> MARRKCRNRFVKKNGQCNVEFTNMDDWPQRYIADMFTTCVDIRWRYMLLLFSLAFLVSWLLFGLIFWLIALIHGDLENPGGDDTFKPCVLQVNGFVAAFLFSIETQTTIGYGFRCVTEECPLAVFMV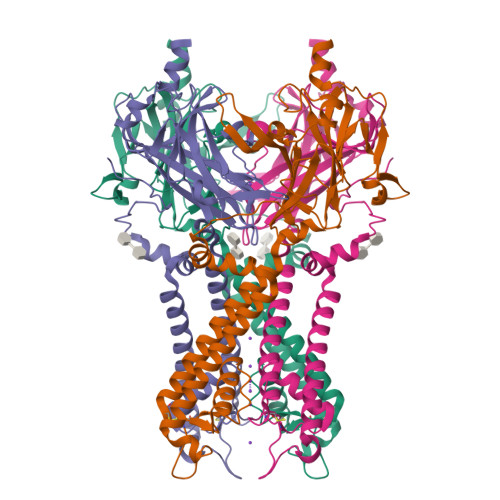VVQSIVGCIIDSFMIGAIMAKMARPKKRAQTLLFSHNAVVAMRDGKLCLMWRVGNLRKSHIVEAHVRAQLIKPRITEEGEYIPLDQIDIDVGFDKGLDRIFLVSPITILHEINEDSPLFGISRQDLETDDFEIVVILEGMVEATAMTTQARSSYLASEILWGHRFEPVLFEEKNQYKVDYSHFHKTYEVPSTPRCSAKDLVENKFLLSNSLEVLFQ> GPHMGGSMQKVSLRVTPRLVLEVNRHNAICVATNVPEFYNARGDLNIRDLRAHVKARMISSQFCGYVLVSLLDSEDQVDHLNIFPHVFSERMILYKPNNVNLMEMCALLSMIENAKSPSIGLCREVLGRLTLLHSKCNNLDSLFLYNGARTLLSTLVK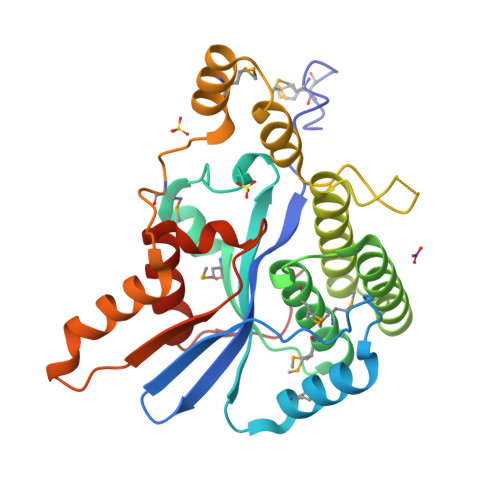YHDLEEGAATPGPWNEGLSLFKLHKELKRAPSEARDLMQSLFLTSGKMGCLARSPKDYCADLNKEEDANSGFTFNLFYQDSLLTKHFQCQTVLQTLRRKCLGSDTVSKIIP> GSHMMRSPYEYHHDLGMNYTLIRDELIVGSQPQKPEDIDHLKQEQNVAYILNLQQDKDIEYWGIDLDSIVRRCKELGIRHMRRPAKDFDPLSLRS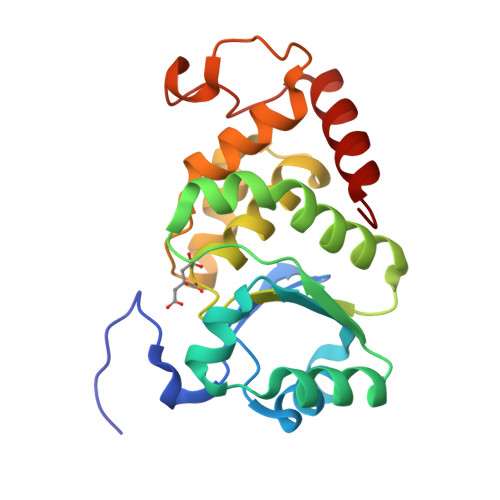QLPKAVSSLEWAVSEGKGRVYVHCSAGLGRAPGVSIAYMYWFCDMNLNTAYDTLVSKRPCGPNKGAIRGATYDLAKNDPWKEPFESLPENAFEDIADWERKLIQERVRALRGT Dibekacin 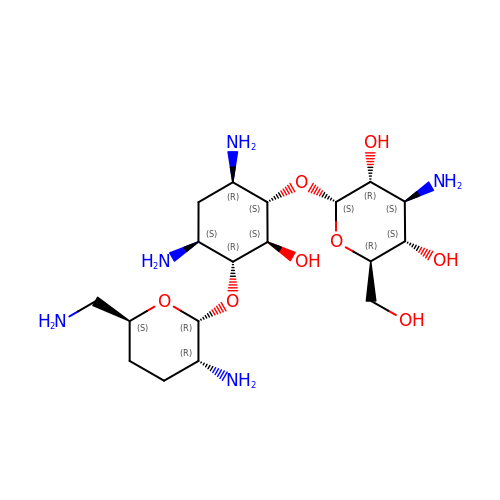| C18 H37 N5 O8 | JJCQSGDBDPYCEO-XVZSLQNASA-N>MERKHHFVLVHNACHGAWIWYKLKPLLESAGHRVTAVELAASGIDPRPIQAVETVDEYSKPLIETLKSLPENEEVILVGFSFGGINIALAADIFPAKIKVLVF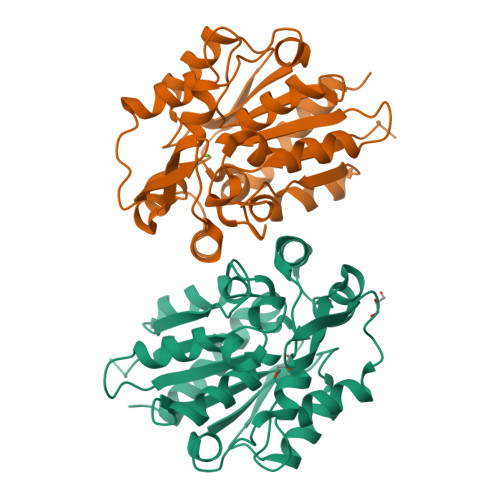LNAFLPDTTHVPSHVLDKLMEMFGGWGDTEFSSHETRNGTMSLLKMGPKFMKARLYQNCPIEDYELAKMLHRQGSFFTEDLSKKEKFSEEGYGSVQRVYVMSSEDKIIPCDFIRWMIDNFNVSKVYEIDGGDHMVMLSKPQKLFDSLSAIATDYMGL[2x]> MGNASSIVQTINVTGDGNVFKPSAETSSTAVPSLSLSPGMLNPGGVPWIAIGDETSVTSPGALRRMTSKDIPETAIINTDNSSGAVPSESALVPYNDEPLVVVTEHAIANFTKAEMALEFNREFLDKLRVLSVSPKYSDLLTYVDCYVGVSARQALNNFQKQVPVITPTRQTMYVDSIQAALKALEKWEIDLRVAQTLLPTNVPIGEVSCPMQSVVKLLDDQLPDDSLIRRYPKEAAVALAKRNGGIQWMDVSEGTVMNEAVNAVAASALAPSASAPPLEEKSKLTEQAMDLVTAAEPEIIASLVPVPAPVFAIPPKPADYNVRTLKIDEATWLRMIPKTMGTLFQIQVTDNTGTNWHFNLRGGTRVVN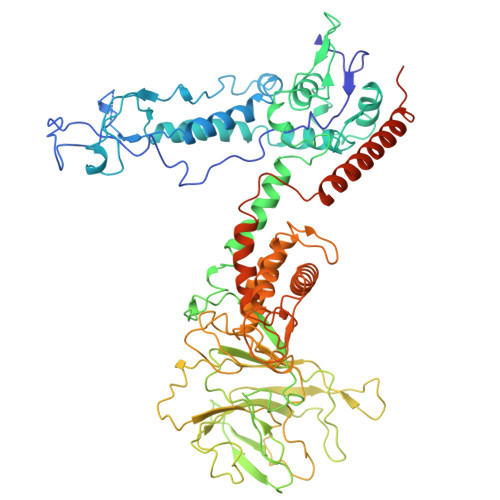LDQIAPMRFVLDLGGKSYKETSWDPNGKKVGFIVFQSKIPFELWTAASQIGQATVVNYVQLYAEDSSFTAQSIIATTSLAYNYEPEQLNKTDPEMNYYLLATFIDSAAITPTNMTQPDVWDALLTMSPLSAGEVTVKGAVVSEVVPAELIGSYTPESLNASLPNDAARCMIDRASKIAEAIKIDDDAGPDEYSPNSVPIQGQLAISQLETGYGVRIFNPKGILSKIASRAMQAFIGDPSTIITQAAPVLSDKNNWIALAQGVKTSLRTKSLSAGVKTAVSKLSSSESIQNWTQGFLDKVSTHFPAPKPDCPTNGDGSEPSARRVKRDSYAGVVKRGYTR>GCUCCUAGUACGAGAG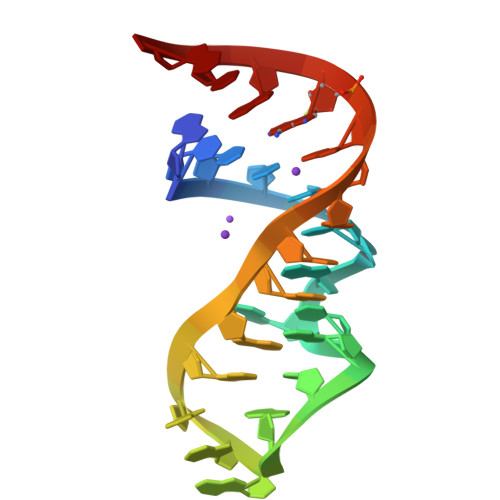GACCGGAGUG[3x]>[2x]GKQGRRFDAQQYLVTSAQALERHYSRNGLYPASQSLANSPYYSFSYTP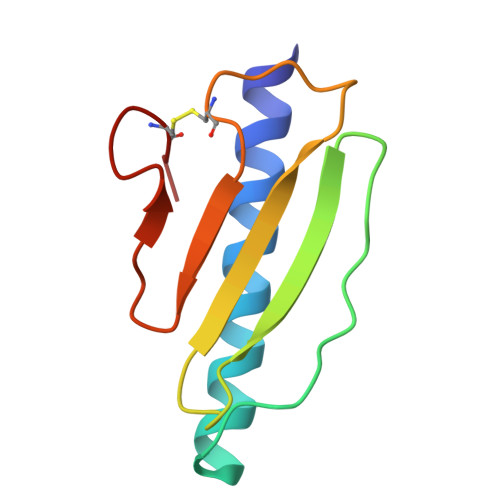TADKFGFSLKAVPTNRQSDPCGTLSLDHKGVRVPATNCWSH Bacillus sp. AHU2216 α-glucosidase (BspAG13_31A), belonging to the glycoside hydrolase family 13 subfamily 31, specifically cleaves α-(1→4)-glucosidic linkages and shows high disaccharide specificity. BspAG13_31A has three domains common to GH13 enzymes: domain A, a catalytic domain that adopts a (β/α)8-barrel fold; domain B, a long loop connecting the third β-strand and third α-helix of domain A (β→α loop 3); domain C, a domain formed by two antiparallel β-sheets that follows domain A. The maltose moiety of G3 and maltotetraose (G4), covering subsites +1 and +2 of this enzyme, adopts a less stable conformation than the global minimum energy conformation, presumably because of steric hindrance by Asn258 at subsite +2. We solved the crystal structures of inactive double mutants, E256Q/N258G and E256Q/N258P, in which the general acid/base catalyst Glu256 was substituted with Gln together with the mutation at Asn258, in complex with G3.

Crystals of E256Q/N258G and E256Q/N258P were prepared by co-crystallization in the presence of 5 mM G3 and G4, respectively, and the structures of E256Q/N258G and E256Q/N258P were solved at 1.7 Å and 1.5 Å resolutions, respectively. In the analysis of the co-crystal of E256Q/N258P and G4, the electron density of only three d-glucosyl residues covering subsites from –1 to +2 was observed. Structural analysis of E256Q/N258G and E256Q/N258P in complex with G3 revealed that the conformation of the maltose moiety bound at subsites +1 and +2 of the double-mutant enzymes was different from that of E256Q. Torsion angles of d-glucosyl residues in subsites +1 and +2 of E256Q/N258G and E256Q/N258P were close to the torsion angles of d-glucosyl residues in the stable α-glucan: Φ (5-O, 1-C, 4′-O, 4′C) = 102° and Ψ (1-C, 4′O, 4′-C, 5′-C) = –120°, which is considered the global minimum energy structure. A molecular mechanics study of maltose suggested that torsion angles of d-glucosyl residues at subsite +1 and +2 in the E256Q-G3 complex are less stable than the global minimum, and the conformation of G3 observed in E256Q/N258G and E256Q/N258P is predicted to be more thermodynamically stable than that in E256Q. This conformational difference of G3 presumably arises from the elimination of steric hindrance by Asn258. The orientation of the side chain of Phe282 in E256Q/N258G, E256Q/N258P, and E256Q differed, presumably because of the closely located amino acid residue at position 258 (Gly, Pro, and Asn in E256Q/N258G, E256Q/N258P, and E256Q, respectively). In the E256Q/N258P-G3 complex, interactions between Phe282 and the d-glucosyl residue in subsite +2 are absent, whereas these interactions were observed in E256Q/N258G and E256Q. Moreover, any additional interactions through the N258P mutation were not observed at subsite +2. Therefore, the stabilized conformation of G3 likely enhanced trisaccharide specificity rather than increasing the enzyme–substrate interaction.

> MEKKWWKEAVAYQIYPRSFMDSNGDGIGDIQGVISKLDYLSDLGIDVIWICPIYQSPNDDNGYDISDYKDIMKDFGTMEDFDELLDEVHHRGMKLIMDLVINHTSDEHPWFLESRSAKENPYRDYYIWHEGKDGKEPNNWESIFSGSAWEFDEKTKEYYMHVFSKKQPDLNWENEKVRHELYEMVNWWLDKGIDGFRVDAISHIKKVAGFPDLPNPEKLDYVPSFEGHMNRPGIQEHLKELKEKTFAKYDIMTVGQAPGVTSDSADEWVAEDGGNFNMIFQFEHMGLWDKGEEKPLDLIELKTILTNWQNGLEKINGWNALYLENHDQIRSVNKFGSTAYRVESAKCLAALYFLMKGTPFIYQGQELGMTNVKFDSIDDYDDVGMINYYRIQREKGDSHDEIMKVIWETGRDNSRTPMQWNTEKNAGFSTGNPWMKVNPNYVDINVEEQKSDKNSVLNFYKQLIKIRKQHDVLVYGTYKLLAEEDSAIYAYTRTLEGKTAVVICNMSPNNQTFEFPSESSFTNIEVLIHNYPLDKNETLEQCTLHPYETRVYLLSLEHHHHHH>ANPLYQK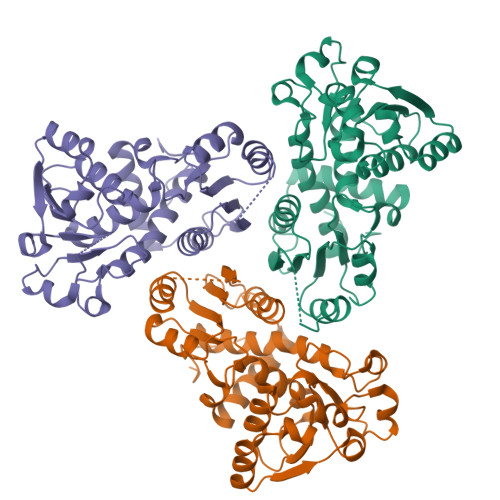HIISINDLSRDDLNLVLATAAKLKANPQPELLKHKVIASCFFEASTRTRLSFETSMHRLGASVVGFSDSANTSLGKKGETLADTISVISTYVDAIVMRHPQEGAARLATEFSGNVPVLNAADASNQHPTQTLLDLFTIQETQGRLDNLHVAMVGDLKYGRTVHSLTQALAKFDGNRFYFIAPDALAMPQYILDMLDEKGIAWSLHSSIEEVMAEVDILYMTRVQKERLDPSEYANVKAQFVLRASDLHNAKANMKVLHPLPRVDEIATDVDKTPHAWYFQQAGNGIFARQALLALVLNRDLVL[6x]>AGGGYWHTSGREILDANNVPVRIAGINWFGFETCNYVVHGLWSRDYRSMLDQIKSLGYNTIRLPYSDDILKPGTMPNSINFYQMNQDLQGLTSLQVMDKIVAYAGQIGLRIILDRHRPDCSGQSALWYTSSV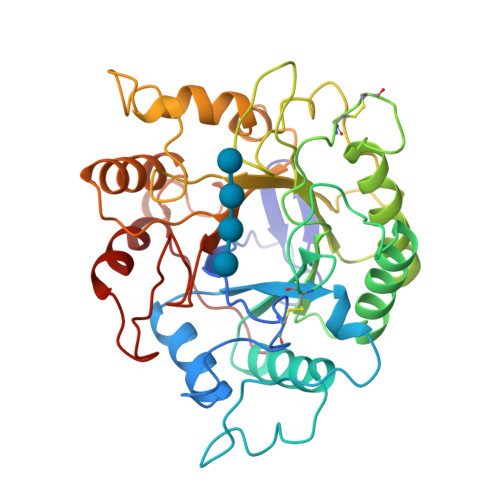SEATWISDLQALAQRYKGNPTVVGFDLHNEPHDPACWGCGDPSIDWRLAAERAGNAVLSVNPNLLIFVEGVQSYNGDSYWWGGNLQGAGQYPVVLNVPNRLVYSAHDYATSVYPQTWFSDPTFPNNMPGIWNKNWGYLFNQNIAPVWLGEFGTTLQSTTDQTWLKTLVQYLRPTAQYGADSFQWTFWSWNPDSGDTGGILKDDWQTVDTVKDGYLAPIKSSIFDPV[2x]>MLAVATITQAEQQDRFLGRGELDELASYFASGAKRLEIAQLLTENSEIIVSRAANRIFQKIENMAKSLRDLSWFLRYATYAIVAGDPNIIVVNTRGLREIIENACSGEATIVALQEIKAASLSYFRK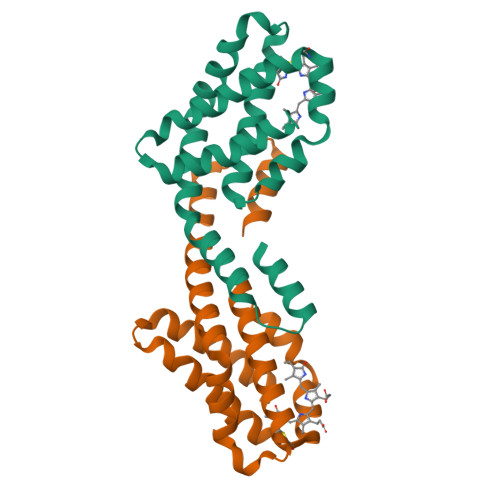DPEAAEIVSQYMDVLITEFKAPLEHHHHHH[2x]> GPHMKTHIDDYSTWDIVKATQYGIYERCRELVEAG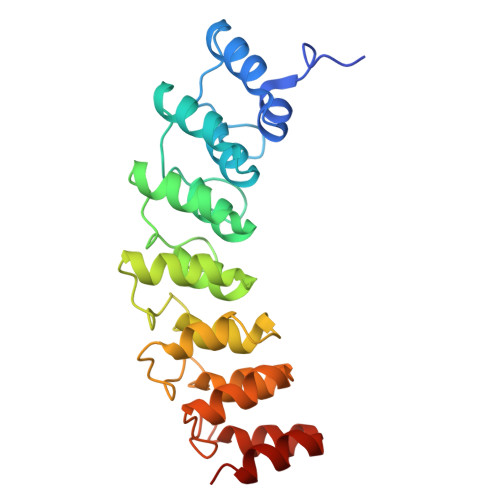YDVRQPDKENVTLLHWAAINNRIDLVKYYISKGAIVDQLGGDLNSTPLHWATRQGHLSMVVQLMKYGADPSLIDGEGCSCIHLAAQFGHTSIVAYLIAKGQDVDMMDQNGMTPLMWAAYRTHSVDPTRLLLTFNVSVNLGDKYHKNTALHWAVLAGNTTVISLLLEAGANVDAQNIKGESALDLAKQRKNVWMINHLQEARQAK>GCGGAAGUAGUUCAGUGGUAGAACACCACCUUGCCAAGG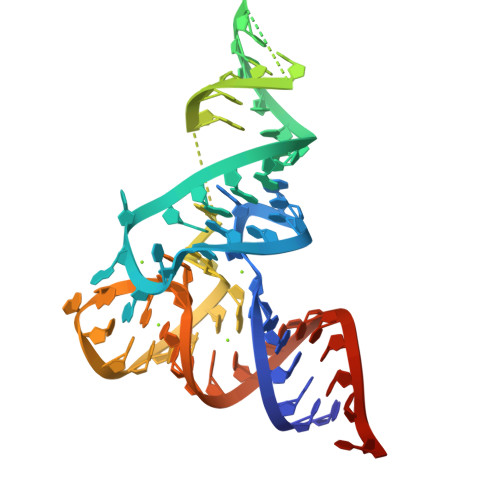UGGGGGUCGCGGGUUCGAGUCCCGUCUUCCGCUCCA[2x]> GAMGSNLKDMEQNSAKAVVLLKAMANERRLQILCMLHNQELSVGELCAKLQLSQSALSQHLAWLRRDGLVTTRKEAQTVYYTLKSEEVKAMIKLLHSLYCEE

HlyU is a conserved transcriptional regulator required for the activation of various virulence genes in Vibrio species. HlyU homologue in Vibrio species is a key regulatory protein that induces the expression of various virulence genes, suggesting that it could be an attractive target to develop the anti-virulence strategies against the pathogenic Vibrios. In the present study, we performed high-throughput screening of 8,385 compounds and identified a small-molecule inhibitor of HlyU, CM14, that significantly inhibited the HlyU activity in V. vulnificus. In conclusion, we identified a small molecule CM14 which inhibits HlyU activity by covalently modifying Cys30 and thus attenuates the virulence of Vibrio species.

The overall structure of the CM14-treated HlyU is similar to that of apo-HlyU. However, there is an extra electron density map around Cys30 of the CM14-treated HlyU suggesting a potential chemical modification of Cys30. Although the moiety attached to Cys30 is partially visible presumably due to the high flexibility, this observation is consistent with the above result that CM14 modifies the Cys30 of HlyU. To this end, tandem mass spectrometric analysis was performed for the CM14-treated HlyU sample. Figure 6a clearly showed that the Cys30 residue (C#) in the HlyU peptide, RLQILC#MLHNQELSVGELCAK, was covalently modified by the moiety with molecular mass of 130.042 Da, indicating that a certain part of CM14, probably consisting of C9H7O, is attached to the Cys30 of HlyU. Notably, further comparison revealed that CM14 induces a conformational change of HlyU, thereby substantially decreasing the distance between Cys30 and Cys96 from 8.4 Å to 4.1 Å. In addition, we found that the distance between two DNA-binding 𝛼-helices (𝛼4) in HlyU dimer by 2.9 Å, which may account for the impaired DNA-binding activity of HlyU. Taken together, the results indicated that CM14 reacts with the thiol group of Cys30 of HlyU via a putative chemical reaction involving Cys96, and consequently inhibits the DNA-binding activity of HlyU. Altogether, the results indicate that CM14-mediated Cys30 modification substantially changes the HlyU conformation, and thus inhibits HlyU binding to target DNA. Biochemical analysis indicated that CM14 prevents HlyU binding to its target promoter DNA. Further mass spectrometric and mutational analyses revealed that a part of CM14 covalently modifies Cys30, a well-conserved residue of HlyU proteins in Vibrio species, both in vitro and in vivo.>MSQPLTTNSVLVEEAAADGDSSAAAPPLFDYHRIDQKLLQNIVYDALVWSTLNCLLVGDKSVQRSGRVPGVGLVHLPLSLLPGPFPESHWKQGCELAPIFNELVDRVSLDGKFLQESLSRTKNADEFTSRLLDIHSKMLQINKKEDIRMGIVRSDYMIDEKTKSLLQIEMNTISTSFALIGCLMTGLHKSLLSQYGKFLGLNSNRVPANNAVDQSAEALAKAWSEYNNPRAAILVVVQVEERNMYEQHYISALLREKHHIRSIRKTLTEIDQEGKILPDGTLSVDGQAISVVYFRAGYTPKDYPSESEWRARLLMEQSSAIKCPTISYHLVGTKKIQQELAKPGVLERFVENKDHIAKLRACFAGLWSLEDSDIVKKAIENPELFVMKPQREGGGNNIYGDELRETLLKLQEAGSQEDAAYILMQRIFPATSPAILVRDGNWDTGHVISEAGIFGTYLRNKDKIIINNESGYMV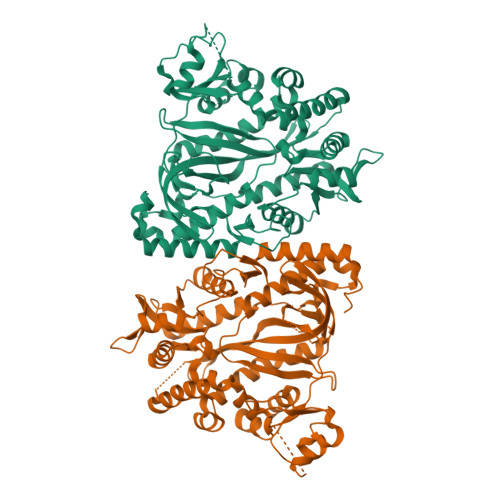RTKISSSYEGGVLPGFGVVDTVYLT[2x]(S)-Fenoprofenoyl-CoA 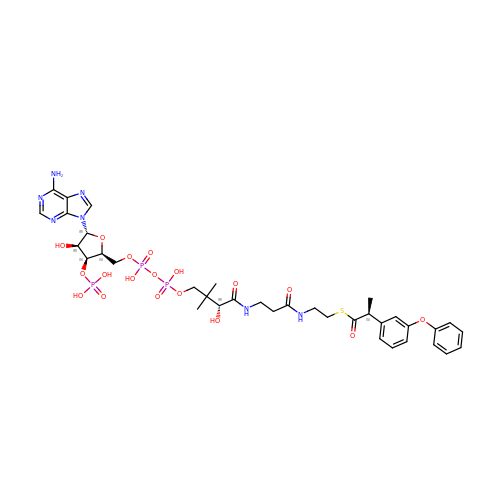| C36 H48 N7 O18 P3 S | OTTFNKHXEHYZEJ-KRDHYROXSA-N>MSKDKVTVITSPSTEELVSLVNSALLEEAMLTIFARCKVHYDGRAKSELGSGDRVIIVKPDGSFLIHQSKKREPVNWQPPGSRVRLELRENPVLVSIRRKPRETLEVELEEVYMVSVFRAEDYEELALTGSEAEMAELIFENPEVIEPGFKPLFREKAIGTGIVAVLGRDSDGNIVVLE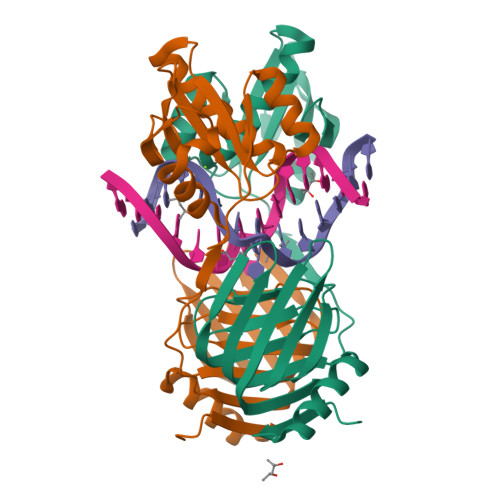LKRRRAELHAVRQLKSYVEILREEYGDKVRGILVAPSLTSGAKRLLEKEGLEFRKLEPPKRDSKKKGRQKTLF[2x]> MLKEFKMIEAVAPDMLDVLQERFQILRNIYWMQPIGRRSLSETMGITERVLRTETDVLKQLNLIEPSKSGMTLTERGLEVYQGLELVMNQLLGMHQIEKEMTQYFGIQRCIVVA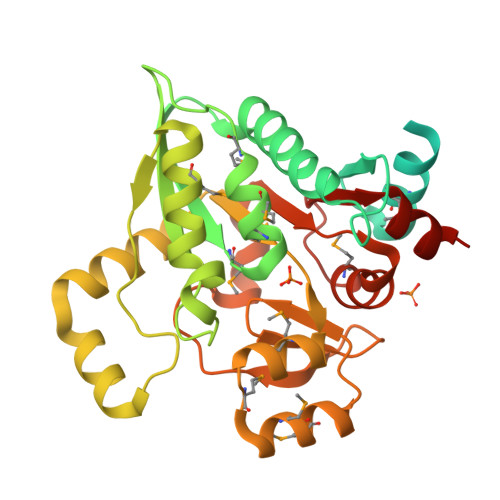GDSDIQKKVLSDFGDVLTNTLNLLLPNGENTIAVMGGTTMAMVAENMGSLETEKRHNLFVPARGGIGEAVSVQANSISAVMANKTGGNYRALYVPEQLSRETYNSLLQEPSIQEVLTLISHANCVVHSIGRALHMAARRKMSDDEMVMLKQKNAVAESFGYFFDEEGKVVYKIPRIGLQLKNLQEIPYVVAIAGGKTKAKAIRAYMKNAPKQTWLITDEAAANEILKGVTL> MMAANPWSPVQPSAASLLLEKCLAAGVLSQNALDQAQLEAPCFSHAEELQRITEIKAEINQKSLELELLRLEKETADITHPLYLGQKHQALQAMNSHLEAVLREKRSLRQRLAQPVCQENLPIEASYHRFTAELLPLAVNFIEKLEIYIKTIQTIPKIPDCASNMDNALMRMESLEAEMEEVTEQILTWREQQKTAFQMNSDANSSCITAQTSYLSIENLH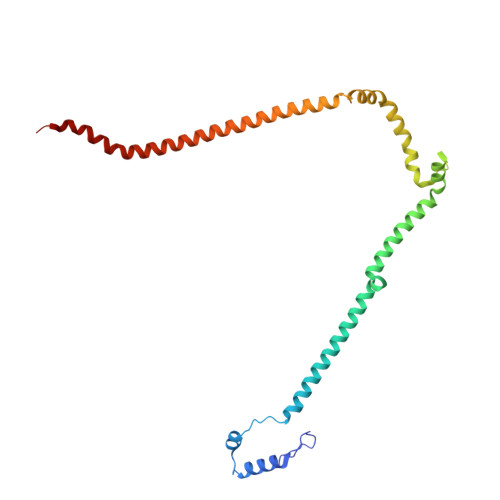P>EKYHQYKINQPEYKAANGKWEIIEFPEKYRQNTIHAALLRTGKVLMVAGSGNNQDNSDDKQYDTRIWDPVKGTIKKVPTPSDLFCTGHTQLANGNLLIAGGTKRYEKLKGDVTKAGGLMVVHNENPDKPITLPAGTKFTGKENGKTFVSKDPVLVPRAEKVFDPATGAFVRNDPGLGRIYVEAQKSGSAYETGTEDNYRVQGLSGADARNTYGIAQKLALDKKDFQGIRDAFEFDPVAEKYIKVDPMHEARAYPTLTTLGDGKILSVSGLDDIGQLVPGKNEVYDPKTKAWTYTDKVRQFPTYPALFLMQNGKIFYSGANAGYGPDDVGRTPGVWDVETNKFTKVPGMSDANMLETANTVLLPPAQDEKYMVIGGGGVGESKLSSEKTRIADLKADDPKFVDGPSLEKGTRYPQASILPDDSVLVSGGSQDYRGRGDSNILQARLYHPDTNEFERVADPLVGRNYHSGSILLPDGR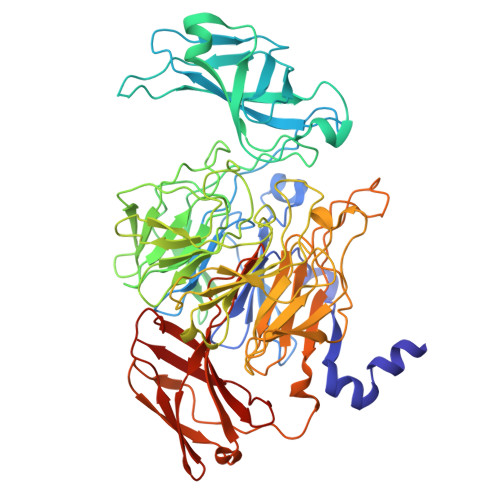LMFFGSDSLYADKANTKPGKFEQRIEIYTPPYLYRDSRPDLSGGPQTIARGGSGTFTSRAASTVKKVRLIRPSASTHVTDVDQRSIALDFKADGDKLTVTVPSGKNLVQSGWYMMFVTDGEGTPSKAEWVRVP[2x]>GTAGKVIKCKAAVLWEQKQPFSIEEIEVAPPKTKEVRIKILATGICRTDDHVIKGTMVSKFPVIVGHEATGIVESIGEGVTTVKPGDKVIPLFLPQCRECNACRNPDGNLCIRSDITGRGVLADGTTRFTCKGKPVHHFMNTSTFTEYTVVDESSVAKIDDAAPPEKVCLIGCGFSTGYGAAVKTGKVKPGSTCVVFGLGGVGLSVIMGCKSAGASRIIGIDLNKDKFEKAMAVGATECISPKDSTKPISEVLSEMTGNNVGYTFEVIGHLETMIDALASCHMNYGTSVVVGVPPSAKMLTYDPMLLFT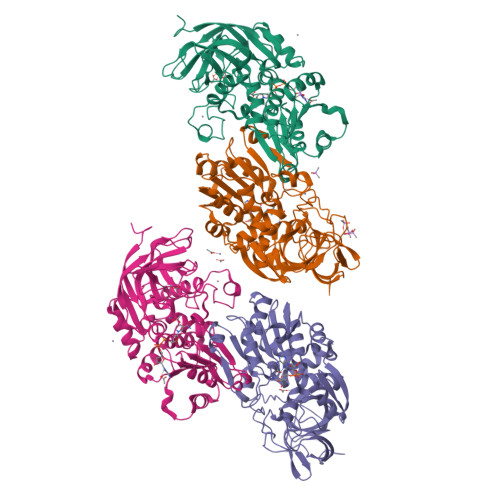GRTWKGCVFGGLKSRDDVPKLVTEFLAKKFDLDQLITHVLPFKKISEGFELLNSGQSIRTVLTF[4x]> DRHHHHHHKLQLGRFWHISDLHLDPNYTVSKDPLQVCPSAGSQPVLNAGPWGDYLCDSPWALINSSLYAMKEIEPKPDFILWTGDDTPHVPNESLGEAAVLAIVERLTNLIKEVFPDTKVYAALGNHDFHPKNQFPAQSNRIYNQVAELWRPWLSNESYALFKRGAFYSEKLPGPSRAGRVVVLNTNLYYSNNEQTAGMADPGEQFRWLGDVLSNASRDGEMVYVIGHVPPGFFEKTQNKAWFRESFNEEYLKVIQKHHRVIAGQFFGHHHTDSFRMFYDNTGAPINVMFLTPGVTPWKTTLPGVVDGANNPGIRIFEYDRATLNLKDLVTYFLNLRQANVQETPRWEQEYRLTEAYQVPDASVSSMHTALTRIASEPHILQRY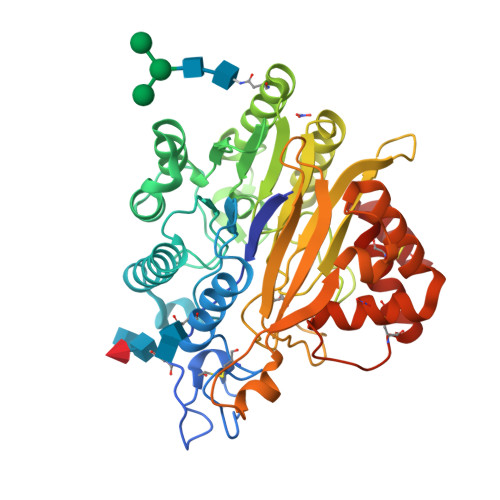YVYNSVSYNHLTCEDSCRIEHVCAIQHVAFNTYATCLHGLGAK>MSPRSRLLASSLRGGLLLRPCSARRSTLLNPSPSPLRKAIFHTTSLRAFKNLAEIATSSKEDASSLKPKGKPSPPGDPLATIEKTAAEQRRADWAIIKQMSRYLWPKDSWSDKARVLLALSLLVGGKVLNVHVPFYFREIIDRLNIDVAAVGGTVSAVAGAVIFAYGASRIGAVVSQELRNAVFSSVAQKAIRRVATQTFGHLLNLDLSFHLSKQTGGLTRAIDRGTKGISYLLTSMVFHIVPTALEIGMVCGILTYQFGWEFAAITAATMAAYTAFTITTTAWRTKFRRQANAADNAASTVAVDSLINYEAVKYFNNEAYEIARYDKALQAYERSSIKVATSLAFLNSGQNIIFSSALTLMMWLGARGVLAGDLSVGDLVLINQLVFQLSVPLNFLGSVYRELRQSLLDMETLFDLQKVNVTIREAPNAKPLALPKGGEIRFENVTFGYYPDRPILRNLSLTIPAGKKVAVVGPSGCGKSTLLRLLFRSYDPQQGKIFIDDQDIKSVTLESLRKSIGVVPQDTPLFNDTVELNIRYGNVNATQEQVIAAAQKAHIHEKIISWPHGYQTRVGERGLMISGGEKQRLAVSRLILKDPPLLFFDQATSALDTHTEQALMANINEVVKEKKRTALFVAHRLRTIYDADLIIVLKEGVVVEQGSHRELMERDGVYAELWMAQEMLHQGEAAEEPAEGEKAEEKK[2x]

Previous studies suggest mitochondrial ABCB7-type exporters are involved in maturation of cytosolic iron-sulfur proteins. Here, we report a series of cryo-electron microscopy structures of a eukaryotic homolog of human ABCB7, CtAtm1, determined at average resolutions ranging from 2.8 to 3.2 Å, complemented by functional characterization and molecular docking in silico. We propose that CtAtm1 accepts delivery from glutathione-complexed iron-sulfur clusters. As anticipated, the architecture of CtAtm1 harbors the classical ABC-fold, packing into a homodimer with six transmembrane segments (TM1–TM6) in each monomer.

To generate an occluded configuration, we again exploited the E603Q form, but this time we supplemented the sample with ATP and cargo, thereby resembling conditions previously exploited to catch such a state of NaAtm130. Then, the cluster in the sample was replaced with GSSG, which permitted us to determine a structure at an average resolution of 2.8 Å, CtAtm1occl. In contrast to previous forms, this sample demonstrates well-defined NBDs in which two ATP molecules are readily identified in the cryo-EM density in proximity to Y450, K480, S481, and Q603. As anticipated, this structure is alike the equivalent state of ScAtm1 and AtAtm3 (RMSD 1.6 and 1.4 Å). Indeed, surface analysis reveals the TM-domain to remain inaccessible from the intermembrane space of mitochondria, but now also from the matrix side. Yet, TM6 remains kinked in the structure, in contrast to occluded states of NaAtm1. In this light, we conclude the structure likely represents an early fully occluded state, triggered by the supplementation of cargo and/or nucleotide. The overall location of the CtAtm1occl pocket across the matrix-membrane interface between TM2, TM3 and TM 6 has essentially not been altered vis-à-vis the matrix-exposed cavity present in the inward-facing conformations, and the highly electropositive surface charge is also maintained. However, interestingly, in the cargo-binding region next to F396, the pocket is divided by residue pairs Y232, V400, and E403 aligning directly each side of the pocket with the two pathways separated by the TM6 linking pairs that are present in our other CtAtm1 structures. Continued passage through the TM-domain is however restricted by the now enlarged inner gate, consisting of H240, F396, and S399.>AQYEDGKQYTTLEKPVAGAPQVLEFFSFFCPHAYQFEEVLHISDNVKKKLPEGVKMTKYHVNFMGGDLGKDLTQAWAVAMALGVEDKVTVPLFEGVQKTQTIRSASDIRDVFINAGIKGEEYDAAWNSFVVKSLVAQQEKAAADVQLRGVPAMFVNGKYQLNPQGMDTSNMDVFVQQYADTVKYLSEKK[2x];>MLRFLNQASQGRGAWLLMAFTALALELTALWFQHVMLLKPCVLCIYERVALFGVLGAALIGAIAPKTPLRYVAMVIWLYSAFRGVQLTYEHTMLQLYPSPFATCDFMVRFPEWLPLDKWVPQVFVASGDCAERQWDFLGLEMPQWLLGI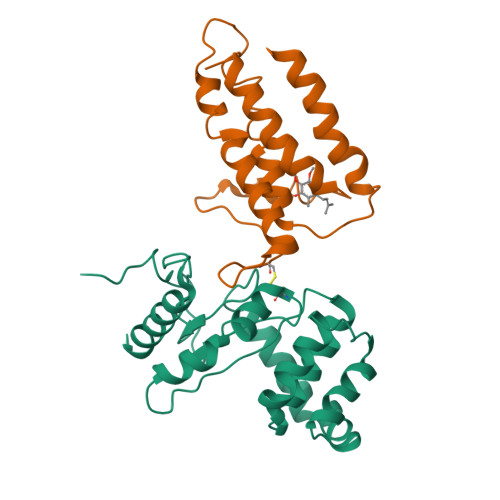FIAYLIVAVLVVISQPFKAKKRDLFGRHHHHHH[2x]>[2x]MHHHHHHENLYFQGGTIYKQFTSRTLLNFFEVAALTDGETNESVAAVCKIAAKDPAIVGVSVRPAFVRFIRQELVKSAPEVAGIKVCAAVNFPEGTGTPDTVSLEAVGALKDGADEIECLIDWRRMNENVADGESRIRLLVSEVKKVVGPKTLKVVLSGGELQGGDIISRAAVAALEGGADFLQTSSGLGATHATMFTVHLISIALREYMVRENERIRVEGINREGAAVRCIGI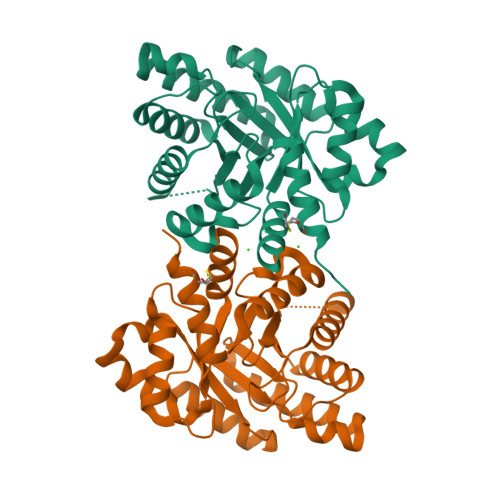KIEVGDVHMAETADFLMQMIFENGPRSIVRDKFRVGGGFNLLKELRDCYESWDSVGVSPDTSP> SMAMFYAHAFGGYDENLHAFPGISSTVANDVRKYSVVSVYNKKYNIVKNKYMWCNSQVNKRYIGALLPMFECNEYLQIGDPIHDLEGNQISIVTYRHKNYYALSGIGYESLDLCLEGVGIHHHVLETGNAVYGKVQHEYSTIKEKAKEMNALKPGPIIDYHVWIGDCVCQVTTVDVH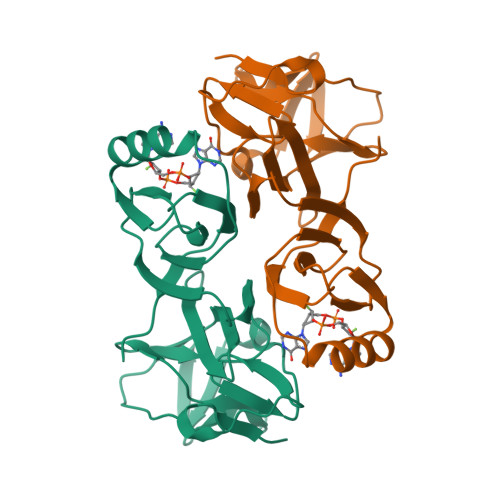GKEIMRMRFKRGAVLPIPNLV>MAPSENYTWKNVRIDGGGFVPGIIFNQKEADLIYARTDIGGAYRWNSATSSWIPLLDWVGWDNWGWNGVMSLATDAADPNRVYAAVGMYTNTWDPNNGAILRSTDRGNTWQATPLPFKVGGNMPGRGMGERLAIDPNRNSIIYYGAEGGNGLWRSTDYGATWAKVSSFTNGGNYAQDPNDPNDYLNKIQGVVWVTFDPASGSAGNTSQVIYVGVADTQNAIYRSTDGGTTWSRLAGQPTGFLPHKGVYDAVNGVLYIAYSDTGGPYDGAKGDVWKFTASSGTWTNISPIPSSSSDLYFGYSGLTIDRKNPNTLMVASQIAWWPDAVFFRSTNGGASWTRIWDWTSYPSRSFRYTMDITEVPWLNFGNSNPVAPEVSPKLGWMNESVEIDPHNSNRLMYGTGATIYATENLTSWDSGGQILLKPMVKGLEETAVLDVVSPPVGAPVYSALGAIGGFRHDDLTKVPTSMYTTPNFSSTTSIDFAELQPATMVRVGNLDSGGGIGVTTNAGGSWWQGQNPPGVTSGGNVALAADGGAIVWAPGGSTNVYLSTTFGSTWTAISA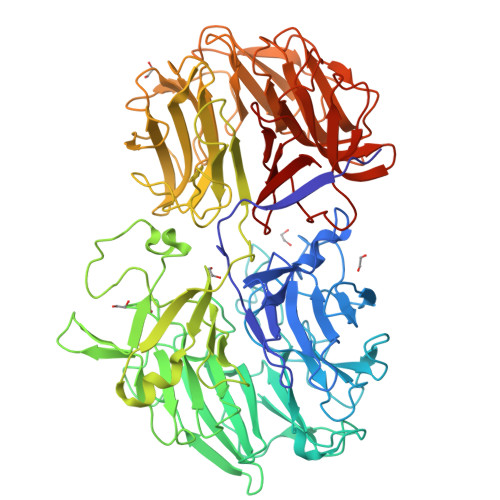LPAGAVIEADRVNPNKFYALANGTFYVSTNKGASFSATVTAGIPAAARKFKAVYGREGDIWLAGGSSTTTYGLWRSTNSGASFTKLASVQEADNVTFGKAATGATYPAIYIIGKVDNVRGVFRSTNEGASWVRINDDQRQYGNFGEAISGDPRIYGRLYLGTNGRGLLYGDSA[2x]> GAGCAGACCAGA;> CGACACTCA;> TCTTCG;> TCTGAGTGGGTCTGC

In this work, we exhaustively probe the ability of all 36 immobile HJ sequences to form DNA crystals in two different designed systems. Three separate self-assembling DNA crystal systems are described in this report: the “4 × 5” and “4 × 6” designs (collectively referred to as the 4 × N systems), and a third construct with a “scrambled” sequence variant of the 4 × 6 lattices. Self-assembly was mediated by three constituent oligonucleotides: (S1) containing four sequence repeats of either 5 or 6 bases; (S2) composed of 21 bases containing complementary regions to both (S1); and (S3) which forms the second junction crossover. The HJ serves as the fundamental component at the core of each unit, and the ultimate assembly of the full lattice is facilitated by the complementary 2-base sticky ends that tail each duplex.

In parallel, we employed the previously reported J1 4 × 6 system (3.05 Å), with P32 symmetry. Seventeen of the 36 junctions successfully crystallized, a 47% success rate. Unlike the 4 × 5 motif, nearly all of the 4 × 6 junction sequences had a strong preference for crystallization in buffers containing ≥2.0 M salts (e.g., LiCl, Li2SO4, KCl, and NaCl), with the majority preferring slightly basic pH conditions in cacodylic acid. The average cell constants for the P32 crystals were a = b = 68.29 Å c = 55.68 Å. The c-axis, in particular, was ~5 Å shorter, and had a much larger degree of variability (σ = 1.97), than those that crystallized using the 4 × 5 motif. The broad range of the short axis spanned from 52.77 to 60.36 Å, and we posit that the flexible axis lengths could be responsible for rendering a larger number of junctions fatal than the 4 × 5 system. However, in the majority of the crystal structures reported here, the cacodylate anion indeed fits best into the electron density map of our X-ray structures, due to the presence of sodium cacodylate in the crystallization solution.>[2x]SSDMAQEPPLTLRERQILKLVAEGKRNRDIAELLSISLKTVETHRLNLMRKLDAHN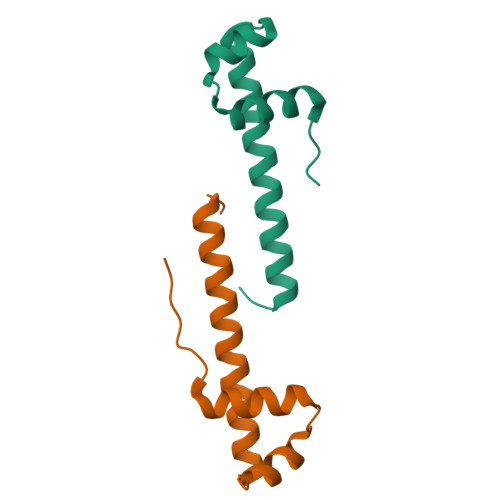AAELSNWARRLGVLEF> SSLPVPYKLPVSLSVGSCVIIKGTPIHSFINDPQLQVDFYTDMDEDSDIAFHFRVRFGNHVVMNRREFGIWMLEETTDYVPFEDGKQFELCIYVHYNEYEIKVNGIRIYG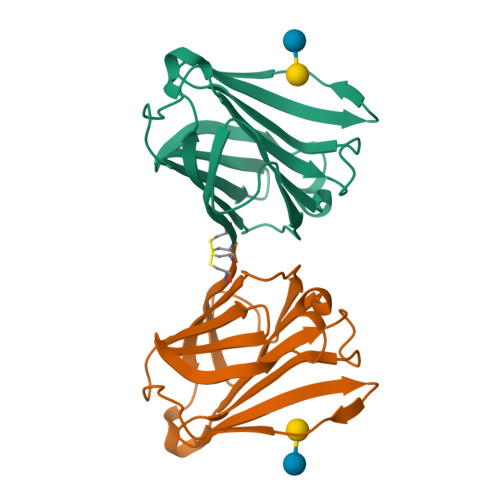FVHRIPPSFVKMVQVSRDISLTSVCVCN>[2x]MARIRVVQGDITEFQGDAIVNAANNYLKLGAGVAGAILRKGGPSIQEECDRIGKIRVGEAAVTGAGNLPVRYVIHAAVLGDEPASLETV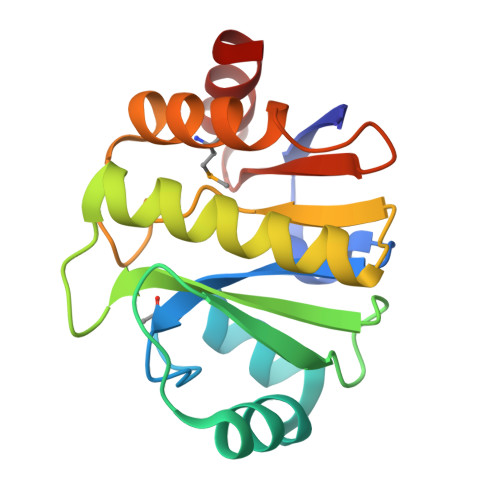RKATKSALEKAVELGLKTVAFPLLGTGVGGLPVEAVARVMLEEIKKAPDTLEVTLYGYREEDAEAIRRAL> MSQSIEEKSVQERTRIKNSRYESGVIPYAKMGYWNPDYQVKDTDVLALFRVTPQPGVDPIEAAAAVAGESSTATWTVVWTDLLTAADLYRAKAYKVDQVPNNPEQYFAYIAYELDLFEEGSIANLTASIIGNVFGFKAVKALRLEDMRLPLAYLKTFQGPATGVILERERLDKFGRPLLGCTTKPKLGLSGKNYGRVVYEALKGGLDFVKDDENINSQPFMRWRERYLFTMEAVNKASAATGEVKGHYLNVTAATMEEMYARANFAKELGSVIIMIDLVIGYTAIQTMAKWARDNDMILHLHRAGNSTYSRQKNHGMNFRVICKWMRMAGVDHIHAGTVVGKLEGDPIITRGFYKTLLLPKLERNLQEGLFFDMEWASLRKVMPVASGGIHAGQMHQLIHYLG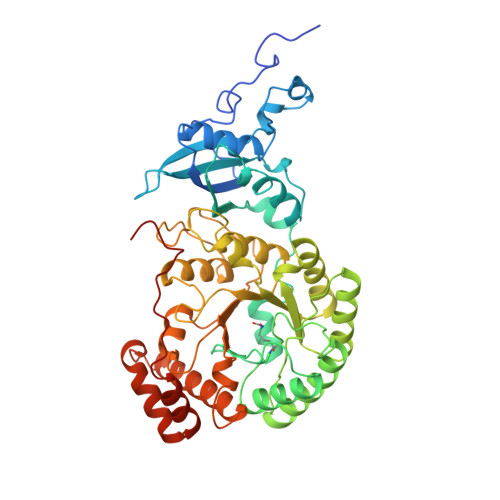EDVVLQFGGGTIGHPDGIQAGATANRVALEAMILARNENRDYLTEGPEILREAAKTCGALRTALDLWKDITFNYTSTDTSDFVETPTANI>MDLTVEPNLHSLITSTTHKWIFVGGKGGVGKTTSSCSIAIQMALSQPNKQFLLISTDPAHNLSDAF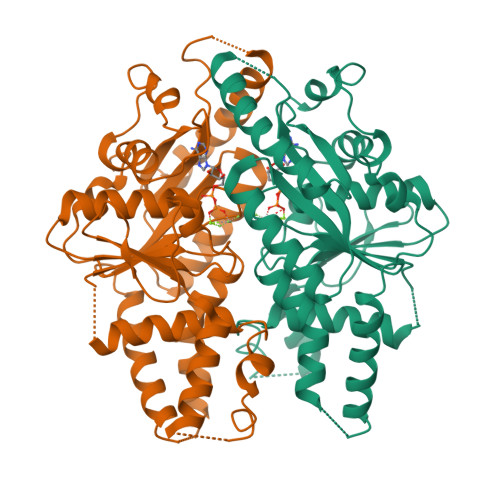GEKFGKDARKVTGMNNLSCMEIDPSAALKDMNDMAVSRANNNGSDGQGDDLGSLLQGGALADLTGSIPGIDEALSFMEVMKHIKRQEQGEGETFDTVIFDTAPTGHTLRFLQLPNTLSKLLEKFGEITNKLGPMLNSFMGAGNVDISGKLNELKANVETIRQQFTDPDLTTFVCVCISEFLSLYETERLIQELISYDMDVNSIIVNQLLFAENDQEHNCKRCQARWKMQKKYLDQIDELYEDFHVVKMPLCAGEIRGLNNLTKFSQFLNKEYNPITDGKVIYELEDKE[4x]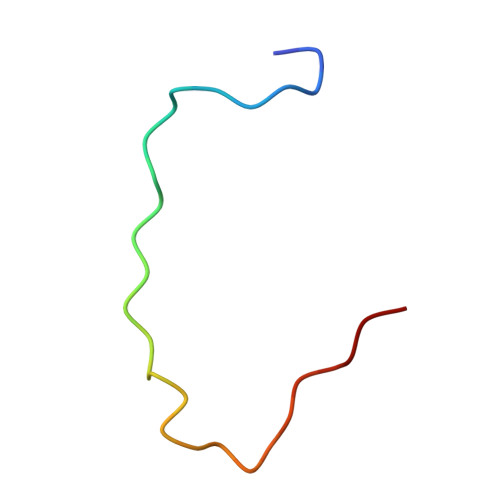> TQSDDDWIPDIQIDPNGLSFNPISDFPDT>AAAAAMVYQVKDKADLDGQLTKASGKLVVLDFFATWCGPCKMIS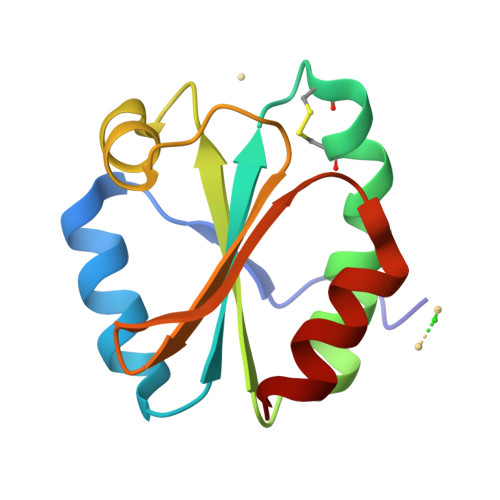PKLVELSTQFADNVVVLKVDVDECEDIAMEYNISSMPTFVFLKNGVKVEEFAGANAKRLEDVIKANI[4x]>MRGSHHHHHHGSITLRGSAEIVAEFFSFGINSILYQRGIYPSETFTRVQKYGLTLLVTTDLELIKYLNNVVEQLKDWLYKCSVQKLVVVISNIESGEVLERWQFDIECDKTAKDDSAPREKSQKAIQDEIRSVIRQITATVTFLPLLEVSCSFDLLIYTDKDLVVPEKWE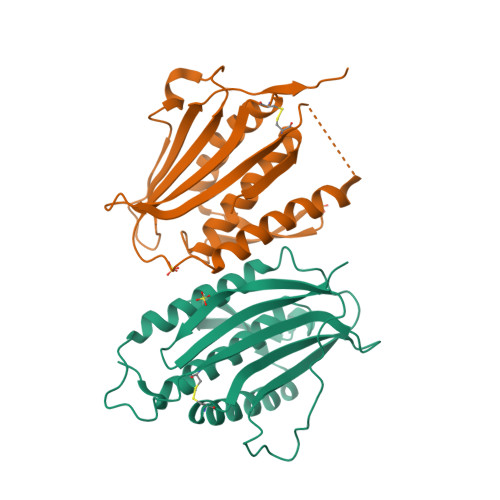ESGPQFITNSEEVRLRSFTTTIHKVNSMVAYKIPVND[12x]>MDRRSFITKAAVGGAAASALAAPALAQSAPKVTWRLASSFPKSLDTIFGGAEVLSKMLSEATDGNFQIQVFSAGELVPGLQAADAVTEGTVECCHTVGYYYWGKDPTFALAAAVPFSLSARGINAWHYHGGGIDLYNEFLSQHNIVAFPGGNTGVQMGGWFRREINTVADMQGLKMRVGGFAGKVMERLGVVPQQIAGGDIYPALEKGTIDAT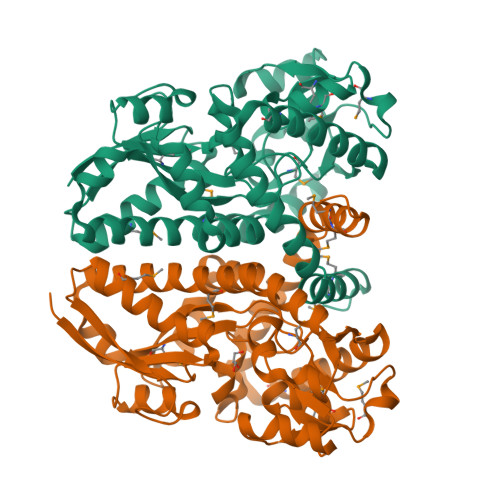EWVGPYDDEKLGFFKVAPYYYYPGWWEGGPTVHFMFNKSAYEGLTPTYQSLLRTACHAADANMLQLYDWKNPTAIKSLVAQGTQLRPFSPEILQACFEAANEVYAEMEASNPAFKKIWDSIKAFRSEHYTWAQIAEYNYDTFMMVQQNAGKL[4x]Acetyl coenzyme A (Ac-CoA)-dependent N-acetylation is performed by arylalkylamine N-acetyltransferase (AANAT) and is important in many biofunctions. Dopamine N-acetyltransferase (Dat) is the first identified insect AANAT from Drosophila melanogaster. Dat exhibits an ordered sequential mechanism in which the cofactor (Ac-CoA) binds first, followed by the binding and acetyl transfer of the substrate. Overall structures revealed that Dat was a globular protein containing a tunnel-like cavity, a substrate located in the middle of the protein, a CoA group located at the bottom, and an acetyl group between the substrate and CoA.

To compare the structures before and after catalysis, two ternary forms, Dat/Ac-CoA/tryptophol (mimicking the enzyme-substrates complex) and Dat/CoA/Ac-TRYP (representing the enzyme-products complex), were obtained through cocrystallization and solved at resolutions of 1.28 and 1.36 Å, respectively. Tryptophol is a dead-end analog of tryptamine for N-acetyltransferase because the amino group in tryptamine is replaced as a hydroxyl group to form tryptophol. The two ternary structures before and after catalysis were very similar (RMSD = 0.65 for all atoms). The backbone carbonyl oxygen of Leu180 may form a hydrogen bond with the active nitrogen atom in Ac-TRYP, while a hydrogen bond with the hydroxyl group of tryptophol was also possible. Therefore, we considered that the role of this hydrogen bond was to position the active nitrogen atom in the substrate. The backbone amide hydrogen of Leu146 also formed a hydrogen bond with acetyl groups either in product (Ac-TRYP) or cofactor (Ac-CoA). We also proposed that the role of this hydrogen bond was to position the acetyl group. In the ternary complexes, Met-aromatic interaction was proposed between Met121 and Tyr64 and between Met121 and Phe114. A bottleneck (the narrowest site) in the cavity surrounded by Met121 and Asp142 was also created after Ac-CoA binding (radius of 1.9 Å) and changed to become wider after substrate binding (radius of 2.4 Å).

> GSHMPYTIELIQPEDGEAVIAMLKTFFFKDEPLNTFLDLGECKELEKYSLKPLPDNCSYKAVNKKGEIIGVFLNGLMRRPSPDDVPEKAADSCEHPKFKKILSLMDHVEEQFNIFDVYPDEELILDGKILSVDTNYRGLGIAGRLTERAYEYMRENGINVYHVLCSSHYSARVMEKLGFHEVFRMQFADYKPQGEVVFKPAAPHVGIQVMAKEV Amlodipine | C20 H25 Cl N2 O5 | 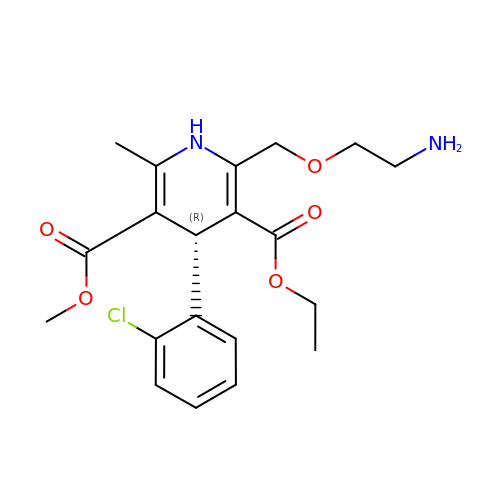HTIQEAQVCYTUBX-QGZVFWFLSA-N2-azanyl-5-[[2-(3-but-3-ynyl-1,2-diazirin-3-yl)ethylamino]methyl]-1,7-dihydropyrrolo[2,3-d]pyrimidin-4-one 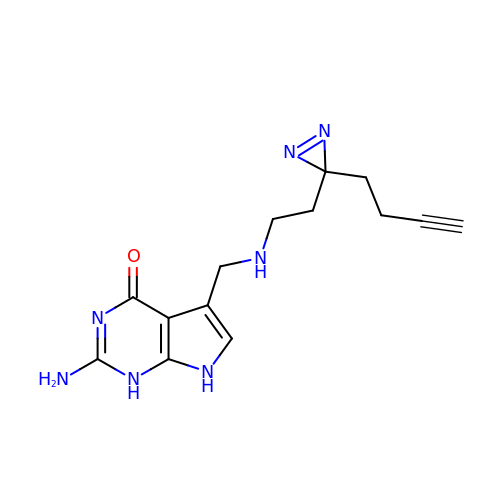| C14 H17 N7 O | XAJHFEIBEFHTRZ-UHFFFAOYSA-N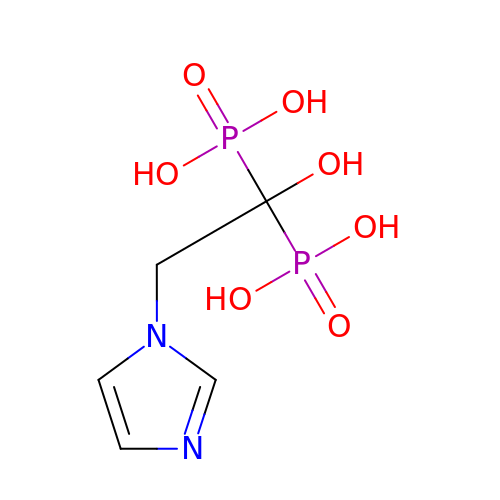ZOLEDRONIC ACID | C5 H10 N2 O7 P2 | XRASPMIURGNCCH-UHFFFAOYSA-N>[3x]SMEEKLKKTNIIFVVGGPGSGKGTQCEKIVQKYGYTHLSTGDLLRSEVSSGSARGKKLSEIMEKGQLV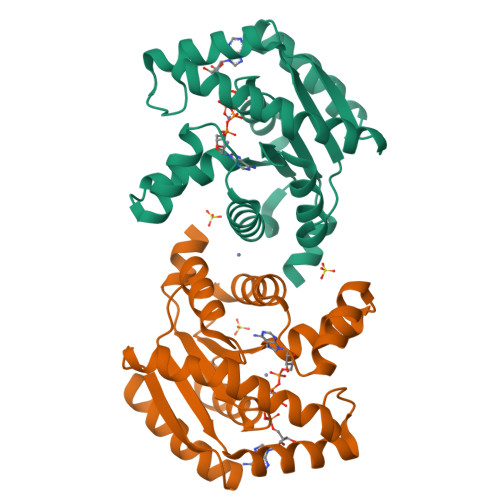PLETVLDMLRDAMVAKVNTSKGFLIDGYPREVQQGEEFERRIGQPTLLLYVDAGPETMTQRLLKRGETSGRVDDNEETIKKRLETYYKATEPVIAFYEKRGIVRKVNAEGSVDSVFSQVCTHLDALLN N-[3-(3-methyl-4-oxo-4,5,6,7-tetrahydro-2H-isoindol-1-yl)-4-phenoxyphenyl]methanesulfonamide | C22 H22 N2 O4 S | 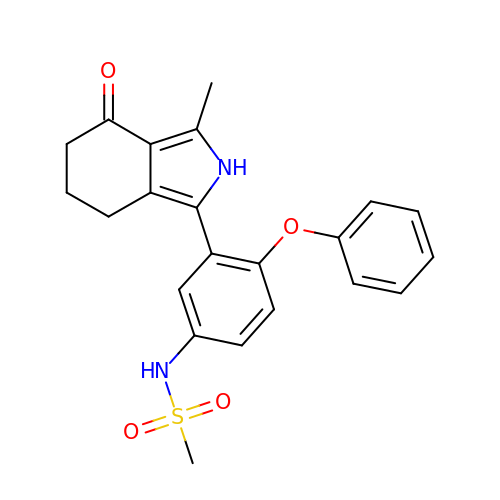GZFJPALDEYOFHA-UHFFFAOYSA-N> ADAPAGTDPRAKWVPQD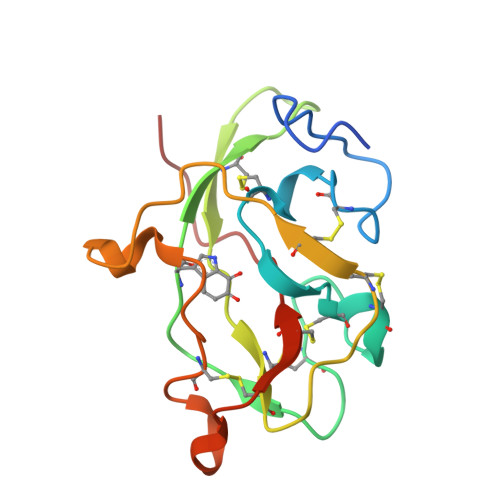NDIQACDYWRHCSIDGNICDCSGGSLTNCPPGTKLATASWVASCYNPTDGQSYLIAYRDCCGYNVSGRCPCLNTEGELPVYRPEFANDIIWCFGAEDDAMTYHCTISPIVGKAS Envelope glycoprotein (Env) trimers derived from the BG505 genotype are the basis of many current HIV vaccine development efforts. When expressed as ectodomain constructs stabilized with SOSIP mutations, trimers based on this clade A sequence can be readily produced at high yields while preserving the native-like, pre-fusion conformation targeted by known broadly neutralizing antibodies (bnAbs). Herein, we introduce cryoelectron microscopy-based polyclonal epitope mapping (cryoEMPEM): a method for rapid, high-resolution structural characterization of antibody-antigen complexes without the need for mAb isolation. Twenty-one high-resolution maps of trimer immune complexes with polyclonal Fabs provided detailed insights to the nature of antibody responses at eight unique epitope clusters predominantly targeted in BG505 SOSIP immunogens.

To explore the effects of nanoparticle presentation of BG505 SOSIP trimers on the epitope specificities of vaccine-elicited antibodies, we used the computationally designed tetrahedral nanoparticle scaffold T33-3154,55. This nanoparticle consists of four copies each of two complementary trimeric components, referred to as T33-31A and T33-31B. Analysis using cryoEM showed that nanoparticles assembled as expected with eight flexibly linked trimer antigens on their surface (top row). Consistent with the structural data, biolayer interferometry (BLI) experiments demonstrated that the antibody binding profiles of BG505 SOSIP fused to each nanoparticle were equivalent to those of free trimers. However, reduced binding to antibodies targeting epitopes in the middle/lower part of the trimer such as the fusion peptide (PGT151, VRC34, and ACS202), gp120–gp41 interface (35O22), gp41–gp41 interface (3BC315), and the trimer base (RM19R and RM20A3) was observed in the context of the assembled nanoparticles. This is likely caused by the crowding of trimer antigens on the nanoparticle surface, limiting the accessibility of epitopes near or at the trimer base; an observation consistent with previously reported data using other nanoparticle scaffolds. While nanoparticle display did not improve the overall levels of NAb responses, it had a dramatic effect on the epitopes targeted and angles of approach of elicited antibodies, particularly after early immunizations. Interestingly, our analyses revealed that presentation on the nanoparticle failed to eliminate base-directed antibody responses, suggesting that this epitope is still readily accessible on the nanoparticle or becomes accessible upon nanoparticle disassembly in vivo.

>[12x]GGEEVVLITVPSALVAVKIAHALVEERLAACVNIVPGLTSIYREEGSVVSDHELLLLVKTTTDAFPKLKERVKELHPYEVPEIVALPIAEGNREYLDWLRENTGLE;>[12x]GSVRGIRGAITVEEDTPAAILAATIELLLKMLEANGIQSYEELAAVIFTVTEDLTSAFPAEAARLIGMHRVPLLSAREVPVPGSLPRVIRVLALWNTDTPQDRVRHVYLNEAVRLRPDLESAQLE>[2x]MSRILAVHASPRGERSQSRRLAEVFLAAYREAHPQARVARREVGRVPLPAVTEAFVAAAFHPQPEQRSLAMQADLALS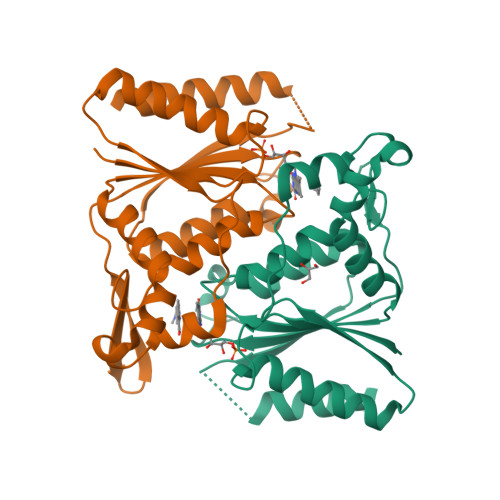DQLVGELFDSDLLVISTPMYNFSVPSGLKAWIDQIVRLGVTFDFVLDNGVAQFRPLLRGKRALIVTSRGGHGFGPGGENQAMNHADPWLRTALGFIGIDEVTVVAAEGEESGGRSFEDSCDEAEQRLLALARSA> MSLDENLIEEIKLADDISKGYNAALNYLSYQLRTRKEVEDKLRSLDIHEDYISEIINKLIDLDLINDKNYAESYVRTMMNTSDKGPKVIKL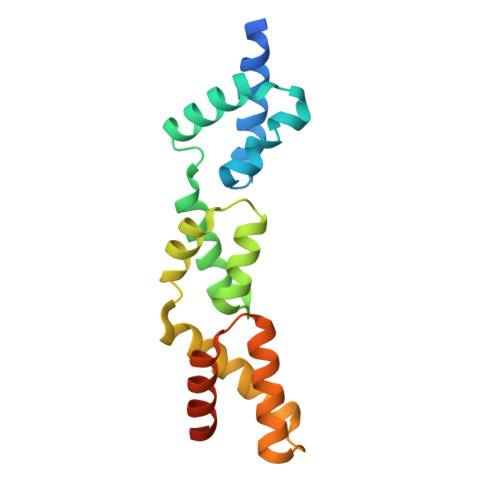NLSKKGIDDNIAEDALILYTDKLQVEKGVTLAEKLANRYSHDSYRNKQNKIKQSLLTKGFSYDIIDTIIQELDLIFDDEGHHHHHH>[2x]MQDGMYQRFLRQHVHPEETGGSDRYCNLMMQRRK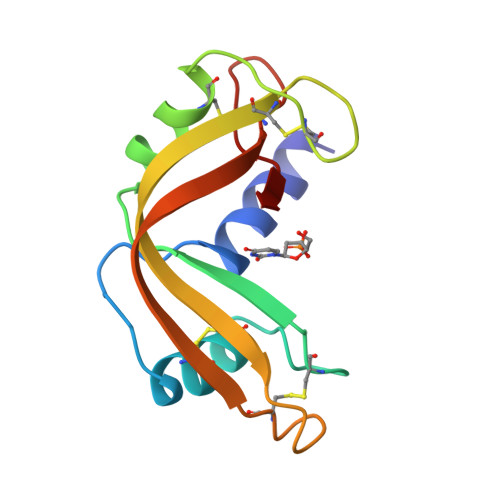MTLYHCKRFNTFIHEDIWNIRSICSTTNIQCKNGKMNCHEGVVKVTDCRDTGSSRAPNCRYRAIASTRRVVIACEGNPQVPVHFDG> MANKRMKVKHDDHYELIVDGRVYYICIVCKRSYVCLTSLRRHFNIHSWEKKYPCRYCEKVFPLAEYRTKHEIHHTGERRYQCLACGKSFINYQFMSSHIKSVHSQDPSGDSKLYRLHPCRSLQIRQYAY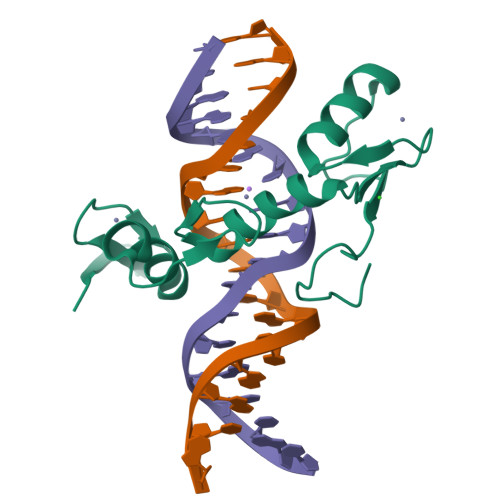LSDRS>PEKSLYEMAVEQFNRAASLMDLESDLAEVLRRPKRVLIVEFPVRMDDGHVEVFTGYRVQHNVARGPAKGGIRYHPDVTLDEVKALAFWMTWKTAVMNLPFGGGKGGVRVDPKKLSRRELERLSRRFFREIQVIIGPYNDIPAPDVNTNADVIAWYMDEYEMNVGHTVLGIVTGKPVELGGSKGREEATGRGVKVCAGLAMDVLGIDPKKATVAVQGFGNVGQFAALLISQELGSKVVAVSDSRGGIYNPEGFDVEELIRYKKEHGTVVTYPKGERITNEELLELDVDILVPAALEGAIHAGNAERIKAKAVVEGANGPTTPEADEIL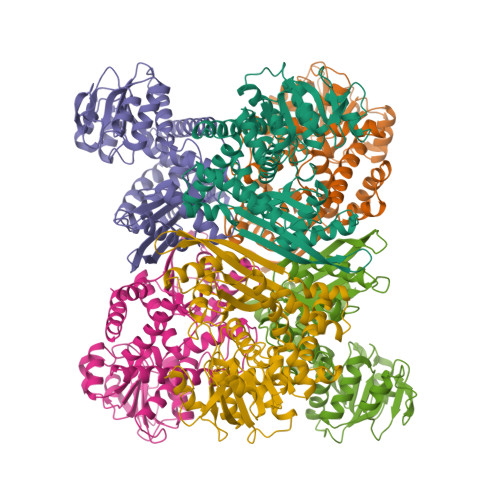SRRGILVVPDILANAGGVTVSYFEWVQDLQSFFWDLDQVRNALEKMMKGAFNDVMKVKEKYNVDMRTAAYILAIDRVAYATKKRGIYP[6x]>[3x]SNAAVSTPVEVAQVEPAAGAVVGVAHPVTVRFAEPVTDRRSAERSLR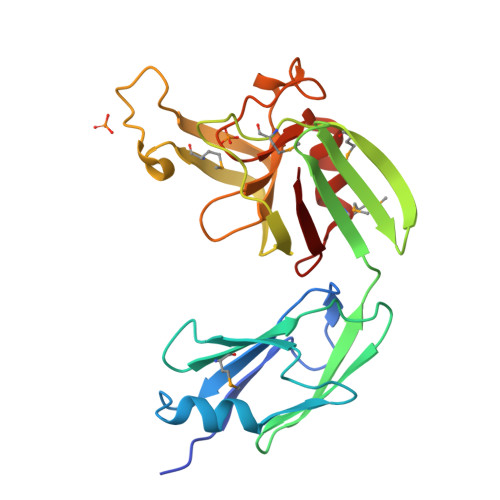IASTDTSAGRFRWPEAAVMEWTPDEFWPAHSTISLSVGGVKTSFNTGAEVLGVADIDAHTFTVSVDGEVLRKMPASMGKPKFPTPRGTFTALAKEPVVVMDSRTIGIPLSDPEGYKLTVNHAVRVTWGGVYVHSAPWSVGSQGYANVSHGCINLSPDNAAWYYDMVSVGDPIIVQA>DKEDEFGYSWKNIQERYGTLTGQLHMIELEKGHSGLGLSLAGNKDRTRMSVFIVGIDPTGAAGRDGRLQIADELLEINGQILYGRS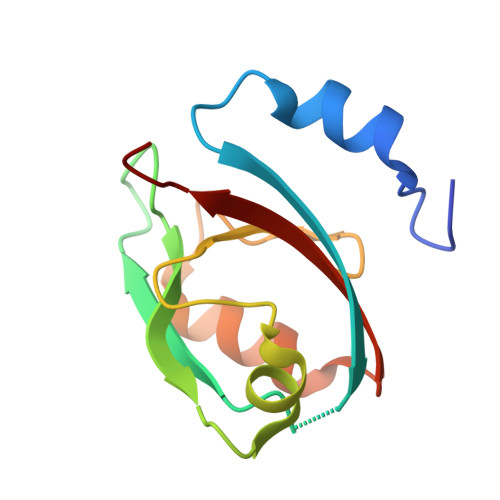HQNASSIIKCAPSKVKIIFIRNADA[4x]>SDKIIHLTDDSFDTDVLKADGAILVDFWAEWCGPCKLIASILDEIADEYQGKLTVAKLNIDQNPGTAPKYGIRGIPTLLLFKNGE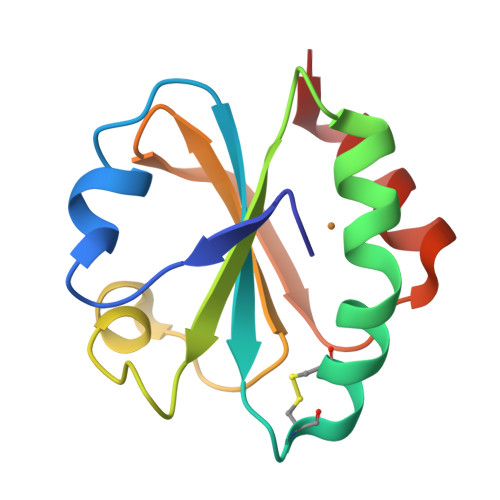VAATKVGALSKGQLKEFLDANLA[2x]> SNAMNLKREQEFVSQYHFDARNFEWENENGAPETKVDVNFQLLQHDQENQVTSLIVILSFMIVFDKFVISGTISQVNHIDGRIVNEPSELNQEEVETLA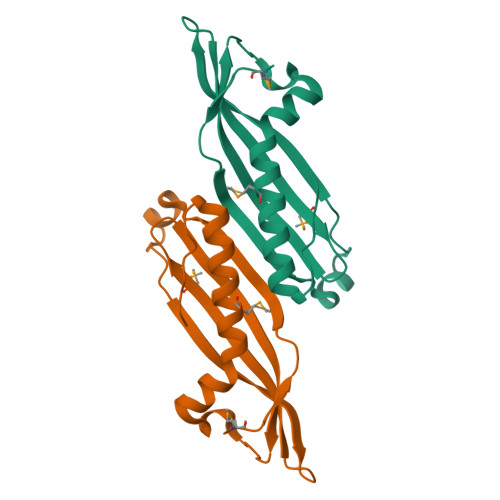RPCLNMLNRLTYEVTEIALDLPGINLEF> MKTEWPELVGKSVEEAKKVILQDKPEAQIIVLPVGTIVTM;> EYRIDRVRLFVDKL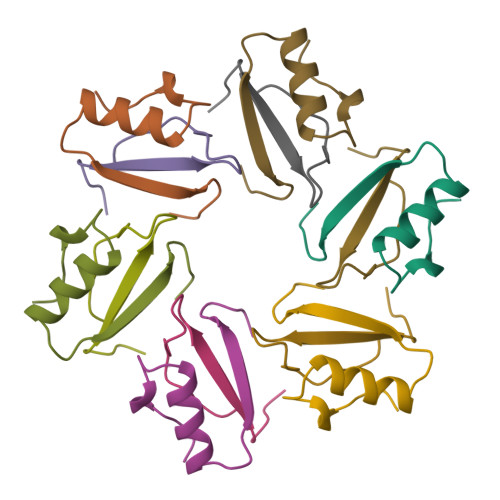DNIAQVPRVG> MKHHHHHHSAGLEVLFQGPGTGSEFELMMFGKKKNNGGSSTARYSAGNKYNTLSNNYALSAQQLLNASKIDDIDSMMGFERYVPPQYNGRFDAKDIDQIPGRVGWLTNMHATLVSQETLSSGSNGGGNSNDGERVTTNQGISGVDFYFLDEEGGSFKSTVVYDPYFFIACNDESRVNDVEELVKKYLESCLKSLQIIRKEDLTMDNHLLGLQKTLIKLSFVNSNQLFEARKLLRPILQDNANNNVQRNIYNVAANGSEKVDAKHLIEDIREYDVPYHVRVSIDKDIRVGKWYKVTQQGFIEDTRKIAFADPVVMAFAIATTKPPLKFPDSAVDQIMMISYMIDGEGFLITNREIISEDIEDFEYTPKPEYPGFFTIFNENDEVALLQRFFEHIRDVRPTVISTFNGDFFDWPFIHNRSKIHGLDMFDEIGFAPDAEGEYKSSYCSHMDCFRWVKRDSYLPQGSQGLKAVTQSKLGYNPIELDPELMTPYAFEKPQHLSEYSVSDAVATYYLYMKYVHPFIFSLCTIIPLNPDETLR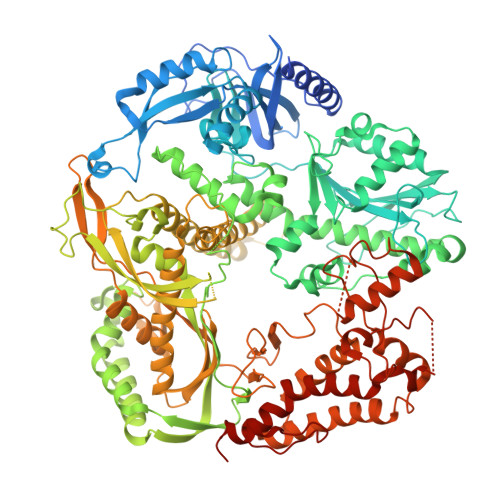KGTGTLCEMLLMVQAYQHNILLPNKHTDPIERFYDGHLLESETYVGGHVESLEAGVFRSDLKNEFKIDPSAIDELLQELPEALKFSVEVENKSSVDKVTNFEEIKNQITQKLLELKENNIRNELPLIYHVDVASMYPNIMTTNRLQPDSIKAERDCASCDFNRPGKTCARKLKWAWRGEFFPSKMDEYNMIKRALQNETFPNKNKFSKKKVLTFDELSYADQVIHIKKRLTEYSRKVYHRVKVSEIVEREAIVCQRENPFYVDTVKSFRDRRYEFKGLAKTWKGNLSKIDPSDKHARDEAKKMIVLYDSLQLAHKVILNSFYGYVMRKGSRWYSMEMAGITCLTGATIIQMARALVERVGRPLELDTDGIWCILPKSFPETYFFTLENGKKLYLSYPCSMLNYRVHQKFTNHQYQELKDPLNYIYETHSENTIFFEVDGPYKAMILPSSKEEGKGIKKRYAVFNEDGSLAELKGFELKRRGELQLIKNFQSDIFKVFLEGDTLEGCYSAVASVCNRWLDVLDSHGLMLEDEDLVSLICENRSMSKTLKEYEGQKSTSITTARRLGDFLGEDMVKDKGLQCKYIISSKPFNAPVTERAIPVAIFSADIPIKRSFLRRWTLDPSLEDLDIRTIIDWGYYRERLGSAIQKIITIPAALQGVSNPVPRVEHPDWLKRKIATKEDKFK> MERYENLFAQLNDRREGAFVPFVTLGDPGIEQSLKIIDTLIDAGADALELGVPFSDPLADGPTIQNANLRAFAAGVTPAQCFEMLAIIREKHPTIPIGLLMYANLVFNNGIDAFYARCEQVGVDSVLVADVPVEESAPFRQAALRHNIAPIFICPPNADDDLLRQVASYGRGYTYLLSRSGVVGAENRGALPLHHLIEKLKEYHAAPALQGFGISSPEQVSAAVRAGAAGAISGSAIVKIIE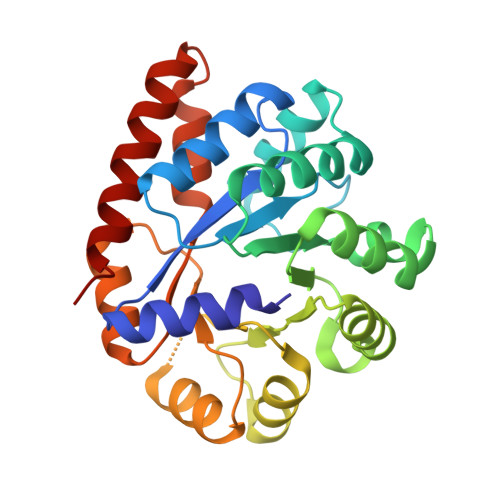KNLASPKQMLAELRSFVSAMKAASRA(2~{R},3~{R},4~{S},5~{S},6~{R})-2-[(2~{R},3~{S},4~{R},5~{R},6~{R})-6-(cyclohexylmethoxy)-2-(hydroxymethyl)-4,5-bis(oxidanyl)oxan-3-yl]oxy-6-(hydroxymethyl)oxane-3,4,5-triol | C19 H34 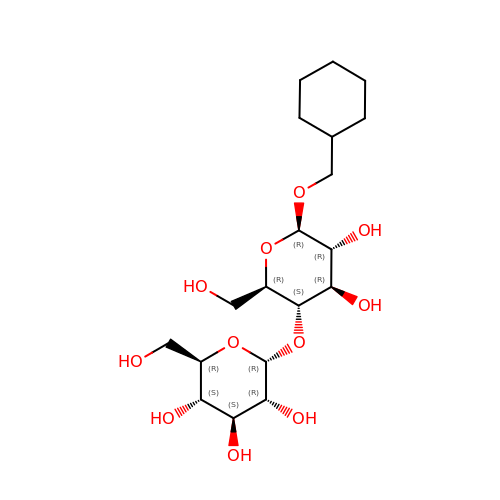O11 | BBUKPWNPDDHXDR-CRINDFDSSA-N>[4x]GAMGSRHRRNGNFESSRLLYSSMSRSIDVACSDADLANFIQENFKKRECVFFTKDTKSMGNLCKCGYPENQHIEGTQVNTTEKWNYKKHTKELPTDAFGDIQFENLGKRGKYIRLSCDTDSETLYDLMTQHWHLKTPNLVISVTGGAKNFALKPRMRKIFSRLIYIAQSKGAWIFTGGTHYGLMKYIGEVVRDNTISRSSEENVVAIGIAAWGMISNRETLIRTADSDGSFLARYIMDDLKRDPLYCLDNNHTHLLLVDNGTHGHPTTEAKVRTQLEKYISERVIPESNYGGKIPIVCFAQGGGKETLKSINVAIKSKIPCVVVEGSGRIADVIASLVEAEGTLASSCVKESLLRFLPRTISRLSEEETESWIKWIKEVLESPHLLTVIKIEEAGDEIVSNAISFALYKAFSTNEHDRDNWNGQLKLLL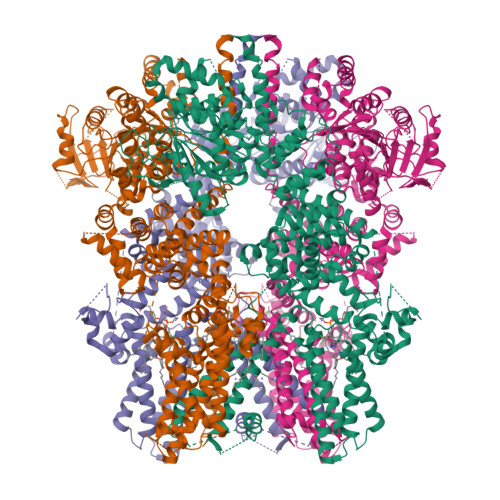EWNQLDLASDEIFTNDRNWESADLQDVMFTALVKDRPKFVRLFLENGLNLRKFLTTEVLRELYTNNFSSLVFKNLQIAKNSYNDALLTFVWKMVEDFRRGFKRDYKNSKDEMEIQLSEECPITRHPLQALFIWSVLQNKKELSKVIWEQTRGCTLAALGASKLLKSMAKVKNDINAAGESEELANEYETRAVELFTECYSNDEDLAEQLLTYSCEAWGGSNCLELAVEARDQQFIAQPGVQNFLSKQWYGEISRDTKNWKIIMCLFFFPLIGCGFISFRKKPVEKSKKLFLYYVSFFTSPFVVFSWNVIFYIAFLLLFAYVLLMDFQKEPTALEIILYVLVFVLLCDEVRQWYMNGSKYFSDLWNVMDTLAIFYFIAGIVFRLHSDESSWYSGRVIFCLDYIVFTLRLIHIFTVSRNLGPKIIMLQRMMIDVFFFLFLFAVWMVAFGVARQGILRKNEHRWEWIFRSVIYEPYLAMFGQYPDDIDGTTYNFDRCTFSGNESKPLCVELDANNQPRFPEWITIPLVCIYMLSTNILLVNLLVAMFGYTVGSVQENNDQVWKFQRFFLVQEYCSRLTIPFPFVIFAYIFMVMRKCFKCCCNKESKEPSICCSRNEDNEILAWEAVMKENYLVKINTKANDSSEEMVHRFRQLDAKLSDLKGLLKEISSKIK6-(4-fluorophenyl)-8-oxidanyl-3-(5-pyrrolo[3,2-c]pyridin-1-ylpentyl)quinazolin-4-one 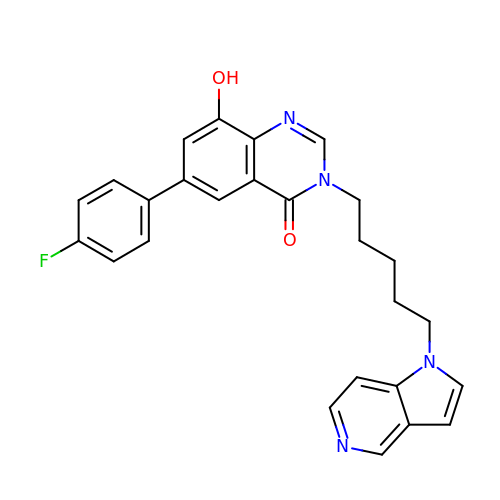| C26 H23 F N4 O2 | GPNCJRAIQDHNTC-UHFFFAOYSA-N>WSHPQFEKSGMAVDTGTEVVYRRPEARDGTRVWELIRDTGSLDLNSPYCYMLLGDYFNDTCMIAEHEGDIVGFISAFRSPRNPETLFVWQVAVASSHRRQGIAKAMLTGLMNQKACHGVRFIETTVSPSNMASRRLFLGYAEEKSIPSTVTVGYGAE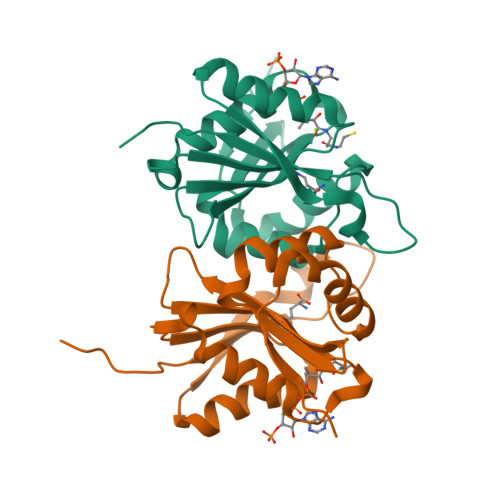MFPDGTTHEDEPLFVIGPFFNDIGSAWSH[2x]>[2x]TC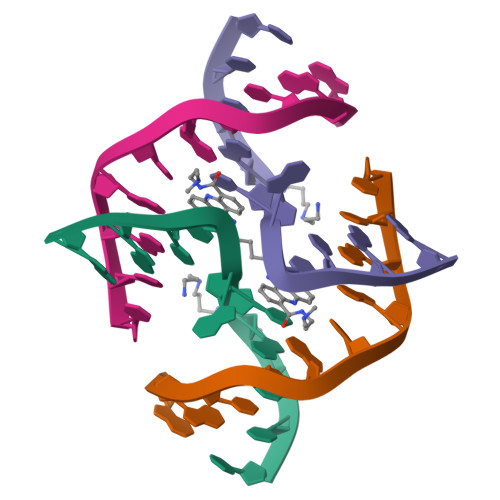GGTACCGA> MVQSMTSVVKAANFILARPTLSKIITPLAQKFTAYAGYREMGLKFNDLLLEETPIMQTAIKRLPSELNYSRNFRILTAHQLALSHQLLPAEKAVKPEEDDNYLIPYILEAEKEAF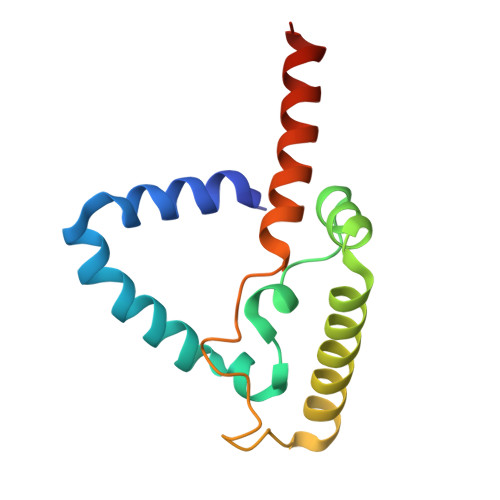EKAELDNIEVKA>[2x]MPIRVPDELPAVNFLREENVFVMTTSRASGQEIRPLKVLILNLMPKKIETENQFLRLLSNSPLQVDIQLLRID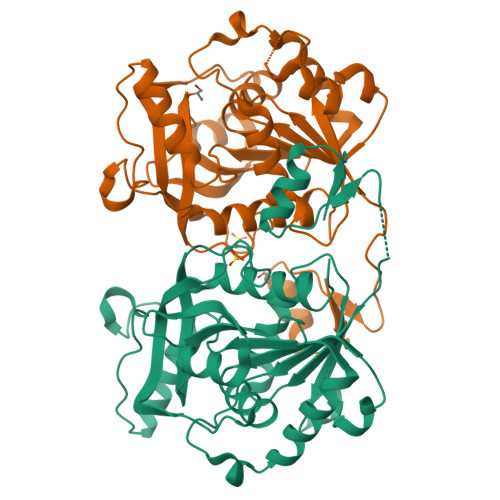SRESRNTPAEHLNNFYCNFEDIQDQNFDGLIVTGAPLGLVEFNDVAYWPQIKQVLEWSKDHVTSTLFVCWAVQAALNILYGIPKQTRTEKLSGVYEHHILHPHALLTRGFDDSFLAPHSRYADFPAALIRDYTDLEILAETEEGDAYLFASKDKRIAFVTGHPEYDAQTLAQEFFRDVEAGLDPDVPYNYFPHNDPQNTPRASWRSHGNLLFTNWLNYYVYQITPYDLRHMNPTLD SpaD, the subject of this report, is the major pilin protein that forms the polymeric backbone, or shaft, of one of the three types of pilus expressed by the human pathogen C. diphtheriae. SpaD is an elongated molecule of ∼125 Å in length built from three tandem domains with Ig-type folds. As in some of the other Gram-positive major pilins, these three domains comprise a single CnaA-type domain flanked by two CnaB-type domains. Two crystal structures, of the full-length three-domain protein at 2.5 Å resolution and of a two-domain (D2-D3) construct at 1.87 Å resolution, show that each of the three Ig-like domains contains a single Lys–Asn isopeptide-bond cross-link, assumed to give mechanical stability as in other such pili.

After testing several different constructs of SpaD, we were able to obtain diffraction-quality crystals from a construct containing residues 27–455, comprising most of the mature full-length SpaD but lacking the C-terminal sortase motif residues. Improved crystals of the full-length native SpaD were then obtained by cryocooling the crystals under high pressure, which enabled data processing to 2.5 Å resolution. The structure was solved by molecular replacement using the structure of the truncated form (SeMet SpaDtryp) as a search model. In the final model, one protomer is complete apart from residues 27–41 (the N-terminus) and 437–439, whereas in the other a large loop between residues 63 and 76, smaller loops between residues 212 and 214 and residues 435 and 436, and the C-­terminal residues 454–455 could not be modelled owing to insufficient density. The angular ‘bend’ between the D1 and D2/D3 domains differs in the two molecules of the asymmetric unit, however. Aside from this, the two copies of SpaD in the asymmetric unit are very similar, with r.m.s.d.s of 0.28 Å between the two D1 domains over 126 Cα atoms and of 0.51 Å between the two D2/D3 domain pairs over 264 Cα atoms. Interpretation of the electron density showed the clear presence of three isopeptide bonds in the structure of SpaD, cross-linking the first and last β-strands of the CnaB-type domains D1 and D3 and the first and second-last strands of the CnaA-type D2 domain. The isopeptide bonds link Lys58 and Asn180 in the D1 domain, Lys187 and Asn299 in the D2 domain and Lys332 and Asn450 in the D3 domain with the essential catalytic acids provided by Glu143, Asp224 and Glu406, respectively. The protein crystals used in the structure determination were from freshly purified SpaD and the three isopeptide bonds seen in the structure must have fully formed during the time taken for crystallization (one to three weeks at 18°C). In our SpaD crystal structure the pilin molecules are stacked end-to-end, bringing the C-terminus of one molecule close to a groove in the N-terminal domain of the next.

>[2x]GPGAVAIAEEGTQVQQTQRANIDFERKGSLTLHKKKGAESEKRATGKEMDDVAGEPLNGVTFKITKLNFDLQNGDWAKFPKTAADAKGHETSTTKEVETSGNGTAVFDNLDLGIYLVEETKAPDGIVTGAPFIVSIPMVNEASDAWNYNVVAYPKNTETKTEKTVKDADQNIQDAYTYTIKADAPTWGKDKKLTAFRFEDELDKRLDFQKVTEVKAGDTVLGTSDYTVNDPATDGNKLVVTLTDEGLKKVKSGDKMSLTFEVKRKEVGNTTELKNRADVIFNNPNTDKEVKNKTNEVVTYHGKLKVVKKDGKEAGKVLKGAEFELYQCTSAAVLGKGPLTVDGVKKWTTGDDGTFTIDGLHVTDFEDGKEAAPATKKFCLKETKAPAGYALPDPNVTEIEFTRAKISEKDKFEGDDEVTLVSEIKNIKQGT> MFDHSFSFDCQDKVILVVEDDYDIGDIIENYLKREGMSVIRAMNGKQAIELHASQPIDLILLDIKLPELNGWEVLNKIRQKAQTPVIML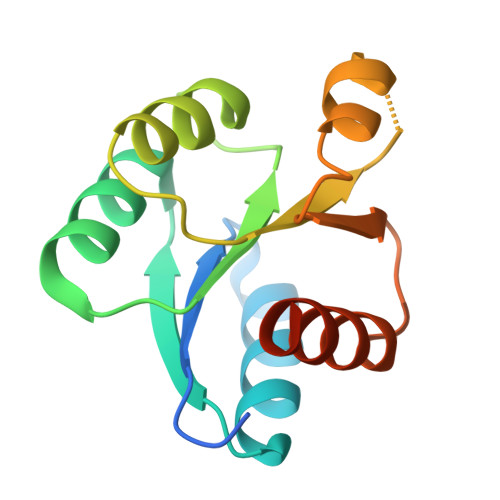TALDQDIDKVMALRIGADDFVVKPFNPNEVIARVQAVLRRTQFANKAT>PPGPPGPPGITGARGLAGPPGPPGPPGPPG[3x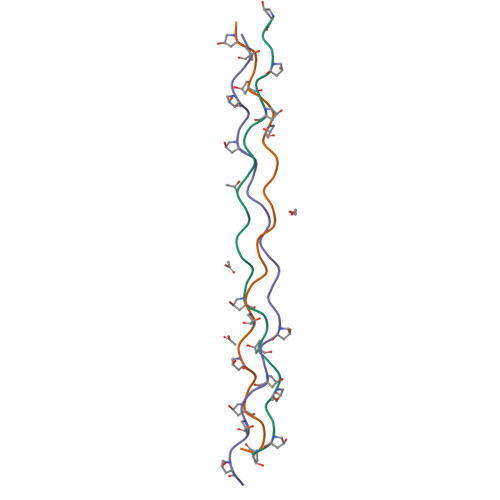]> GPHMRTFF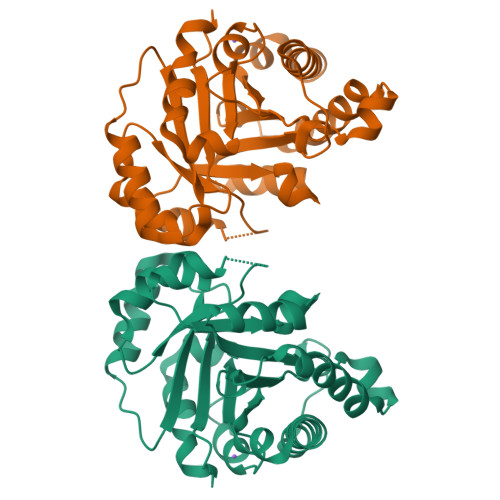VGGNWKANPKTVEEAEKLIEMLNGAKVEGNVEVVVAAPFIFLPTLQQKLRKDWKVSAENVFTKPNGTVPMIKSFGIEWTILGHSERRDILKEDDEFLAAKAKFALENGMKIIYCCGEHLSEREAGKASEFVSAQIEKMIPAIPAGKWDDVVIAYEPIWAIGTGKVASTQDAQEMCKVIRDILAAKVGADIANKVRILYGGSVKPNNCNELAACPDVDGFLVGGASLEPGFINIVNSNVHSK>[6x]MSLHDQRVHAERDPLDPQAHGLTITRIETIPMVAPLAREFRGSHYHMTHRATIVTRVHTDAGIIGEAYTGDEHETMFDIDRIIHEELAPTLIGQDAMAIERLWDSGYKVTFD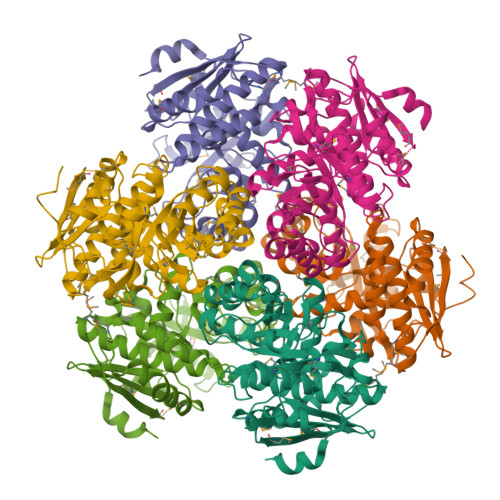ILRDRRLGLVALAAVNTAIWDAVGKALKMPLWKLWGGYRNELPMIAIGGYYGEPLGSIADEMHNYQELGLAGVKFKVGGLSAAEDAARITAAREAAGDDFIICIDANQGYKPAVAVDLSRRIADLNIRWFEEPVEWHNDKRSMRDVRYQGSVPVCAGQTEFSASGCRDLMETGAIDVCNFDSSWSGGPTAWLRTAAIATSYDVQMGHHEEPQVSTHLLASQPHGTIAECFHPDRDPFWWNMITNRPKLNNGTLTLSDRPGLGWDLNWDYIDQYRVSKDEGHHHHHH>[3x]MEAIRKELSRSYQELNEEAEPVAIDPEEAEDEEKEQEEAASAVAPDRDSDRSSPPVRFSRTCLKNFFSVLLILVYLLLMGVAVFLVYQTITDFRDKLKHPVMSVSYKEVNMYDAPGIALYPGKARLLSCEHHWYDHIPPLKDPGQPGENTCVTQDISY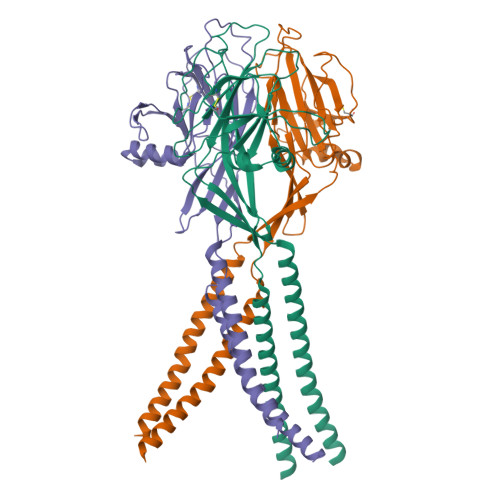IDPYTNKTMKHALIVQGPRDVRRRELVFLQFHLNETKQDFSAIDYLLFSSYEAFLKSHDQVKFMQDCESSFSSWKFSGGFRTWVKMSLVKTKEEDGSQSVEFRQETSVVNFIDRRETPDKGDQLFFVVFEWKDPYIQEIQDIITANPWSMIALLCSVFLVLFKAADFAKLSVKWMIKVRRRHLKKRARELNHIS> MKKMAEFTFEIEEHLLTLSENEKGWTKEINRVSFNGAPAKFDIRAWSPDHTKMGKGITLSNEEFQTM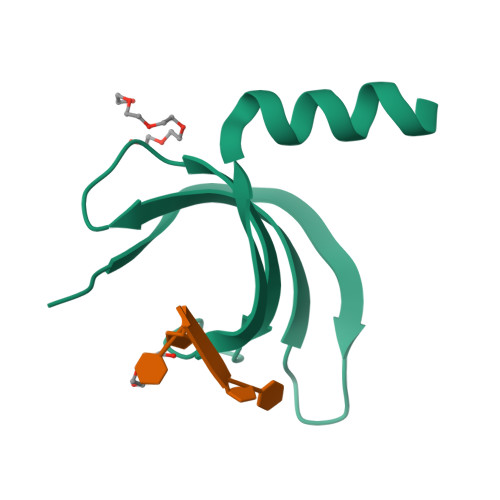VDAFKGNLEHHHHHH> MSGRWSHPQFEKIHQRREAGARETCRDQIKGSDKDEEPSAALSHGQGYRPCGRPARNSKPEAGARPPAVPIMVNDPPVPALLWAQEVGHVLAGRARRLMLQFGVLFCTILLLLWVSVFLYGSFYYSYMPTVSHLSPVHFHYRTDCDSSTASLCSFPVANVSLAKSGRDRVLMYGQPYRVTLELELPESPVNQDLGMFLVTVSCYTRGGRIISTSSRSVMLHYRSQLLQVLDTLLFSSLLLFGFAEQKQLLEVELYSDYRENSYVPTTGAIIEIHSKRIQMYGAYLRIHAHFTGLRYLLYNFPMTCAF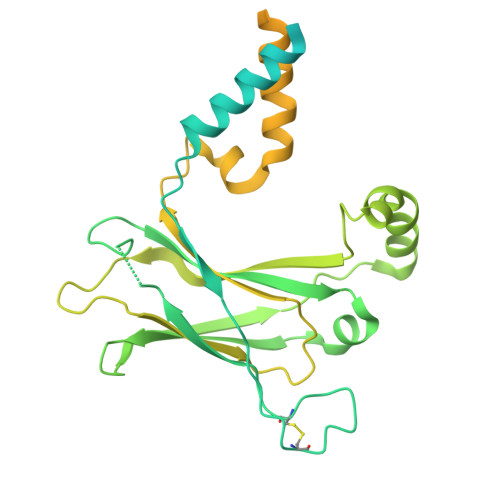VGVASNFTFLSVIVLFSYMQWVWGAVWPRHRFSLQVNIRQRDNSHHGAPRRISRHQPGQESTQQSDVTEDGESPEDPSGTEGQLSEEEKPEKRPLNGEEEQEPEASDGSWEDAALLTEANPPTSASASALAPETLGSLRQRPTCSSS>PLIRIDLTSDRSREQRRAIADAVHDALVEVLAIPARDRFQILTAHDPSDI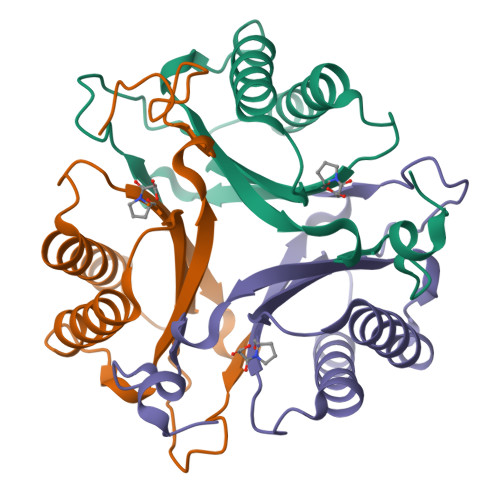IAEDAGLGFQRSPSVVIIHVFTQAGRTIETKQRVFAAITESLAPIGVAGSDVFIAITENAPHDWSFGFGSAQYVTGELAIPATGAA[5x]> DCSSGWSSYEGHCYKVFKQSKTWADAESFCTKQVNGGHLVSIESSGEADFVGQLIAQKIKSAKIHVWIGLRAQNKEKQCSIEWSDGSSISYENWIEEESKKCLGVHIETGFHKWENFYCEQQDPFVCEA;> DCPSDWSSYEGHCYKPFNEPKNWADAENFCTQQHTGSHLVSFQSTE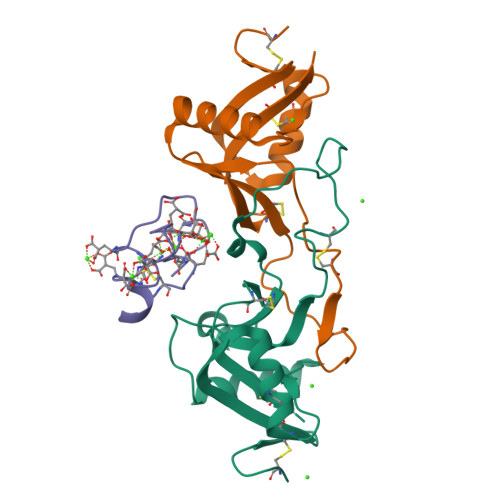EADFVVKLAFQTFDYGIFWMGLSKIWNQCNWQWSNAAMLKYTDWAEESYCVYFKSTNNKWRSITCRMIANFVCEFQA;> ANSFLEEVKQGNLERECLEEACSLEEAREVFEDAEQTDEFWSKY>[3x]MSNPSLVIVSPALPGANNGNWRTAQRWKALLSPVCSARVVQQWPDADASADTVMLALHARRSAESIAHWAHAHPGRGLGVVLTGTDLYQDIGSDPQAQRSLQLAQRLVVLQALGAEALPPECRAKARVVYQSTSARAELPKSARQLRAV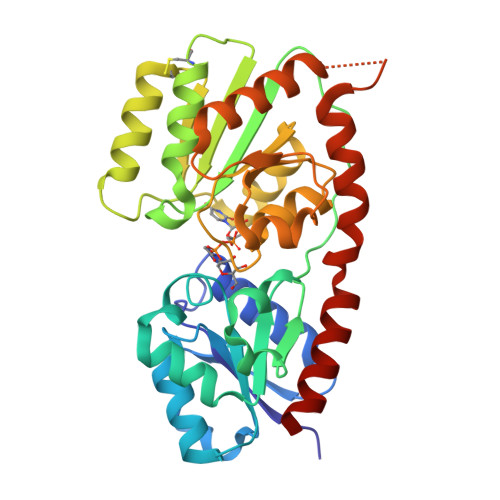MVGHLRQVKSPQTLFDAARLLCGREDIRIDHIGDAGDAGLGELARALASDCPGYRWLGALPHAQTRQRIQRAHVLVHTSALEGGAHVIMEAVRSGTPVLASRVPGNVGMLGNDYAGYFPHGDAAALAALLEACRAGQGSKDRAAGLLDSLRTQCALRAPLFDPRAEQAALFQLLNELQPPPP> MNVDPHFDKFMESGIRHVYMLFENKSVESSEQFYSFMRTTYKNDPCSSDFECIERGAE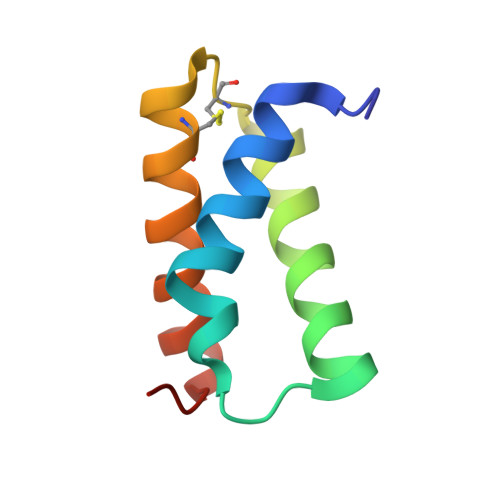MAQSYARIMNIKLETE>MFKDYTREKFAKENFPDLSKHNNVMASQLTYELYEKYWDKVTPNGVTFDKCIQTGVDNPGNKFYGKKTGCVFGDEYSYECYKEFFDKCIEEIHHFKPSDKHPAPDLDHNKLVGGVFEDKYVKSCRIRCGRSVKGVCLPPAMSRAERRLVEKVVSDALGGLKGDLAGKYYPLTTMNEKDQEQLIEDHFLFEKPTGALLTTSGCARDWPDGRGIWHNNEKNFLVWINEEDHIRVISMQKGGDLKAVFSRFARGLLEVERLMKECGHGLMHNDRLGYICTCPTNMGTVVRASVHLRLAFLEKHPRFDEMLGKLRLGKRGTGGESSLATDSTYDISNWARLGKSERELVQVLVDGVNLLIACDKKLEAGQSIDDMIPK[2x];>[2x]MGSAIQDYFVKNRVGHSKPWESGKFKAADNFPDLSKHNNVMASQLTKELYEKYWDKVTPNGVTFDKCIQTGVDNPGNKFYGKKTGCVFGDEYSYECYKEFFDKCIEEIHHFKPSDKHPAPDLDHNKLVGGVFEDKYVKSCRIRCGRSVKGVCLPPAMSRAERRLVEKVVSDALGGLKGDLAGKYYPLTTMNEKDQEQLIEDHFLFEKPTGALLTTSGCARDWPDGRGIWHNNEKNFLVWINEEDHIRVISMQKGGDLKAVFSRFARGLLEVERLMKECGHGLMHNDRLG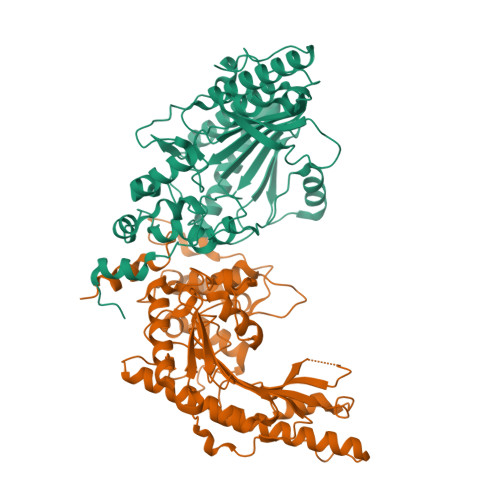YICTCPTNMGTVVRASVHLRLAFLEKHPRFDEMLGKLRLGKRGTGGESSLATDSTYDISNWARLGKSERELVQVLVDGVNLLIACDKKLEAGQSIDDMIPK> SSNFSSERIRYAKWFLEHGFNIIPIDPESKKPVLKEWQKYSHEMPSDEEKQRFLKMIEEGYNYAIPGGQKGLVILDFESKEKLKAW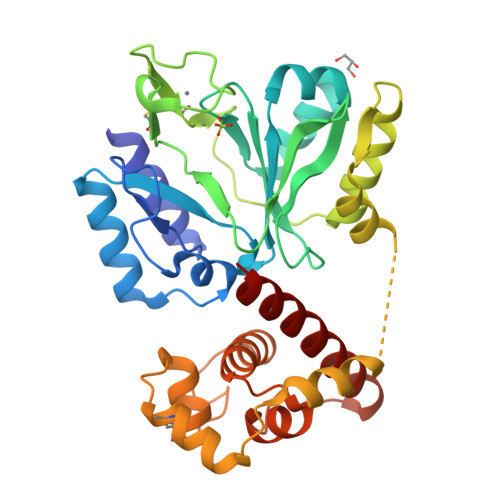IGESALEELCRKTLCTNTVHGGIHIYVLSNDIPPHKINPLFEENGKGIIDLQSYNSYVLGLGSCVNHLHCTTDKCPWKEQNYTTCYTLYNELKEISKVDLKSLLRFLAEKGKRLGITLSKTAKEWLEGKKEEEDTVVEFEELRKELVKRDSGKPVEKIKEEICTKSPPKLIKEIICENKTYADVNIDRSRGDWHVILYLMKHGVTDPDKILELLPRDSKAKENEKWNTQKYFVITLSKAWSVVKKYLEA>MSRHWPLFDLRITTPRLQLQLPTEELCDQLIDTILEGVHDPDRMPFSVPWTRASREDLPFNTLSHLWQQLAGFKRDDWSLPLAVLVDGRAVGVQALSSKDFPITRQVDSGSWLGLRYQGHGYGTEMRAAVLYFAFAELEAQVATSRSFVDNPASIAVSRRNGYRDNGLDRVAREGAMAEALLFRLTRDDWQ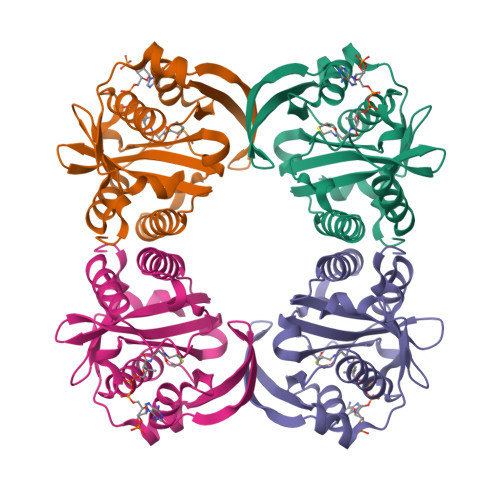RHRTVEVRVDGFDRCRPLFGPLEPPRY[4x]>[15x]VTPGAILVTHPLESYYNQFLDG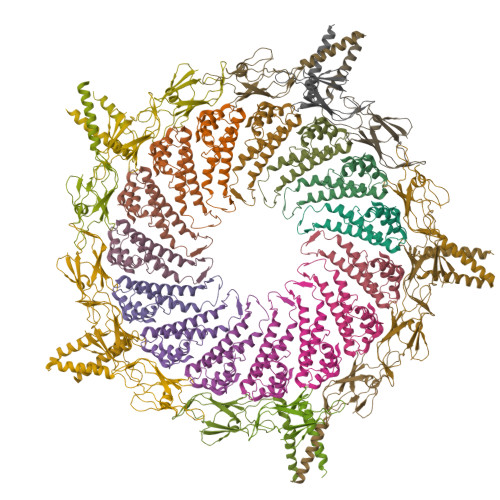LPTSELEELEIEFVAMCIGFPRSQNNFVNALLDLSTIEVYTIRTSVKEILRLDKLNKESIENRQVTKVEDITMNMNYIGDIKDELVTEVKKLARILKLPVLDNLYVSYDDVEGRIGANGLLEPLNRGSGFGSYLTGYTVR;>MRRLKGTIRHLDDQPWINVSLFLTLINGTFNSANQYPIDTKHAKTDQNGEFVFNVVPNVGIDQSYYILTTPDNKKHSFTVPDGTSDIEFSVVREAGIIATDPEYTNVLNYLEDYIDDAIANIQASSVIAEIFTCGQTISALKALRFDSSTGKVFYASSSDATHLNKCVGVSSQSGVLNDNIQVVTSGYLSDQSWNWTIGSPIFFDSGGTLTHTPGSSYYQVIGIPVTTNKVLISVEQPIKL[15x]> MAGKKRRLSQASVLRYYAKRFTMNVGTTAHVLGKEVAGNPWVAKAIDKLSYQETYNWISDYQASHLAKQVAKQVAEKYGIPPTFQGLLMAYAEKVVANYILDYKGESLTQMHDNYLYELMQKMPIAPTGTSSGYIYVFIGKDGKTHTVDMSKVLTDIEDALLKRA;> MAGRQAHRKFDVRNDTSTRWKGKLYGIFVNYMGEDYAKEFVEQAYSNYEKVFVNIYTKIHNQLRTTLTSSAGAGATFPLWQIINEAIYAVYLTHKETASFLYAKYVARGIQPNVVKKILAETGNALKGIVPAVAQELGETVLDESNVISVVDDIVRKNPALPNSYAGIILQEARISTTPH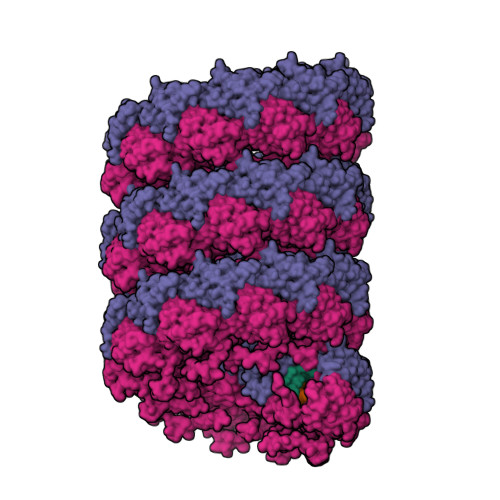YEGTEGFSSMESAYSALEEIEKGL> SGQNHHEVVKFMDVYQRSYCHPIETLVDIFQEYPDEIEYIFKPSCVPLMRCGGCCNDEGLECVPTEESNITMQIMRIKPHQGQHIGEMSFLQHNK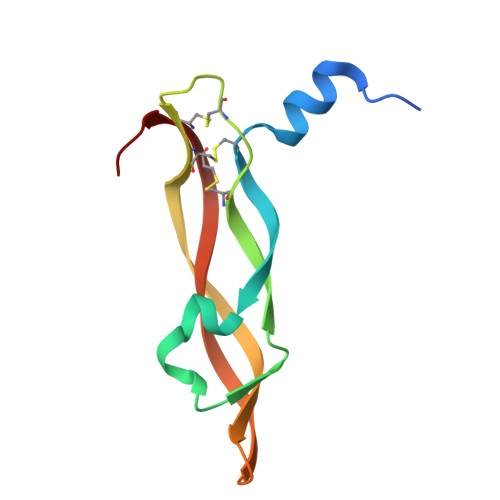CECRPKKD>LEYGKKVNYQQFDNIYLGAEASVVSCFLQDSEGLIWIGSNKGLFSYDGYSTQQHFTYGENNNTRIYCGVIIDNTYLYMGTDNGILVYNYRADRYEQPETDFPTDVRTMALQGDTLWLGALNGLYTYQLQSRKLTSFDTRRNGLPNNTIYSIIRTKDNQIYVGTYNGLCRYIPSNGKFEGIPLPVHSSQSNLFVNSLLEDTTRQCVWIGTEGYLFQYFPSTGQIKQTEAFHNNSIKSLALDGNGDLLAGTDNGLYVYHNDTTPLQHIIHDSRNIQSLTNNIIWNIFADQEHNIWLGTDYGISLSRYNSALQFIPISQITGTGDGNQFYSLFRDSKGFYWFGGANGLIRFTDPAGERHDAIWYRMGDKTYPLSHNRIRHIYEDKEQQLWIATDGSINRYDYATRQFIHYNIVDNTGTYNTNWTYYIFEDTAGQLWISTCLGGIFVVDKHKLMQSTSGQYIAEQNYSVHNGLSGMFINQIIPDNEGNVWVLLYNNKGIDKINPRTREVTKLFADELTGEKSPNYLLCDEDGLLWVGFHGGVMRINPKDESQQSISFGSFSNNEILSMTCVKNSIWVSTTNGLWIIDRKTMDARQQNMTNKRFTSLLF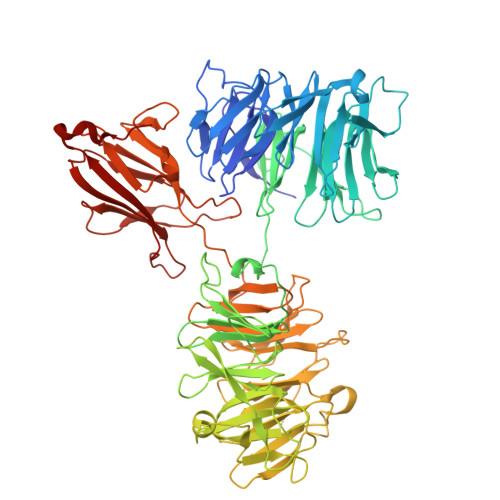DPKEDCVYLGGADGFGISHSNLEATYQPERPILLTALYINNQLVSPRTRDDVPNIRYTNSIKLKYDQNNLSFELSDLPYSLDEKNKFVYRLEGMDKEWNFLKSNINRITYSNLSYGNYQLIISKLERDGQPSNRPHILNIRILPPWLEHHHHHH[2x]> DLDTHFTQYKLARPYI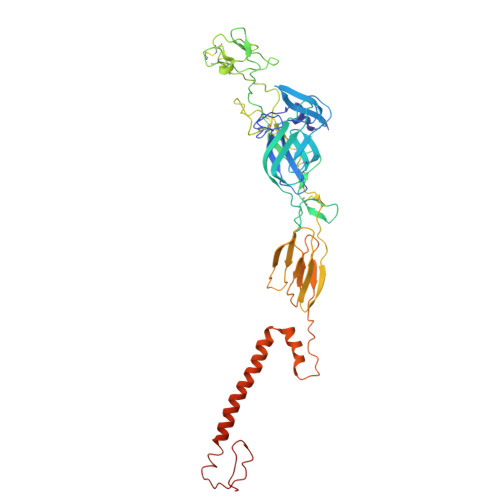ADCPNCGHSRCDSPIAIEEVRGDAHAGVIRIQTSAMFGLKTDGVDLAYMSFMNGKTQKSIKIDNLHVRTSAPCSLVSHHGYYILAQCPPGDTVTVGFHDGPNRHTCTVAHKVEFRPVGREKYRHPPEHGVELPCNRYTHKRADQGHYVEMHQPGLVADHSLLSIHSAKVKITVPSGAQVKYYCKCPDVREGITSSDHTTTCTDVKQCRAYLIDNKKWVYNSGRLPRGEGDTFKGKLHVPFVPVKAKCIATLAPEPLVEHKHRTLILHLHPDHPTLLTTRSLGSDANPTRQWIERPTTVNFTVTGEGLEYTWGNHPPKRVWAQESGEGNPHGWPHEVVVYYYNRYPLTTIIGLCTCVAIIMVSCVTSVWLLCRTRNLCITPYKLAPNAQVPILLALLCCIKPTRA> MEYYKQSKYETYSEIIEKERTARFESVALEQLQIVHISSEADFSAVYSFRPKNLNYFVDIIAYEGKLPSTISEKSLGGYPVDKTMDEYTVHLNGRHYYSNSKFAFLPTKKPTPEINYMY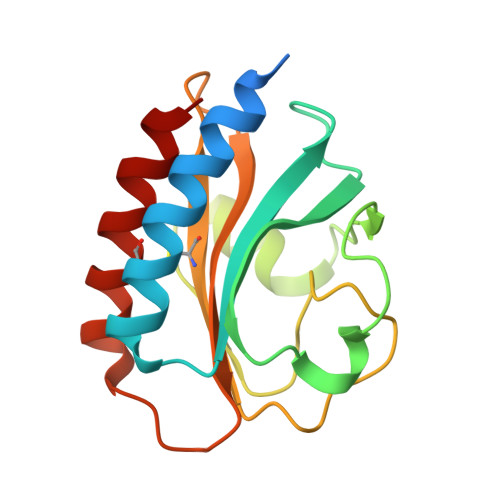SCPYFNLDNIYAGTITMYWYRNDHISNDRLESICAQAARILGRAK> GAQVSTQKTGAHENQNVAANGSTI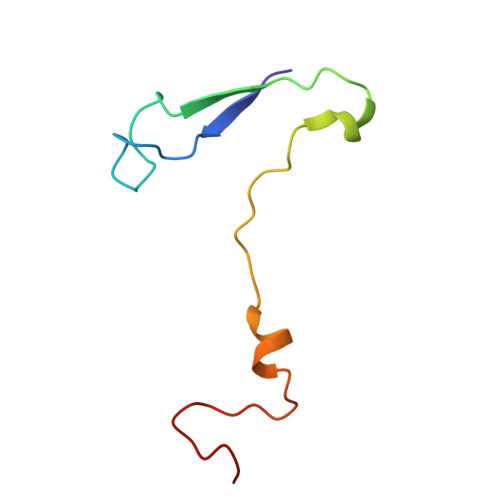NYTTINYYKDSASNSATRQDLSQDPSKFTEPVKDLMLKTAPALN> RSPWEENFSRSYPCDEKKQNDSVIAECSNRRLQEVPQTVGKYVTELDLSDNFITHITNESFQGLQNLTKINLNHNPNVQHQNGNPGIQSNGLNITDGAFLNLKNLRELLLEDNQLPQIPSGLPESLTELSLIQNNIYNITKEGISRLINLKNLYLAWNCYFNKVCEKTNIEDGVFETLTNLELLSLSFNSLSHVPPKLPSSLRKLFLSNTQIKYISEEDFKGLINLTLLDLSGNCPRCFNAPFPCVPCDGGASINIDRFAFQNLTQLRYLNLSSTSLRKINAAWFKNMPHLKVLDLEFNYLVGEIASGAFLTMLPRLEILDLSFNYIKGSYPQHINISRNFSKLLSLRALHLRGYVFQELREDDFQPLMQLPNLSTINLGINFIKQIDFKLFQNFSNLEIIYLSENRISPLVKDTRQSYANSSSFQRHIRKRRSTDFEFDPHSNFYHFTRPLIKPQCAAYGKALDLSLNSIFFIGPNQFENLPDIACLNLSANSNAQVLSGTEFSAIPH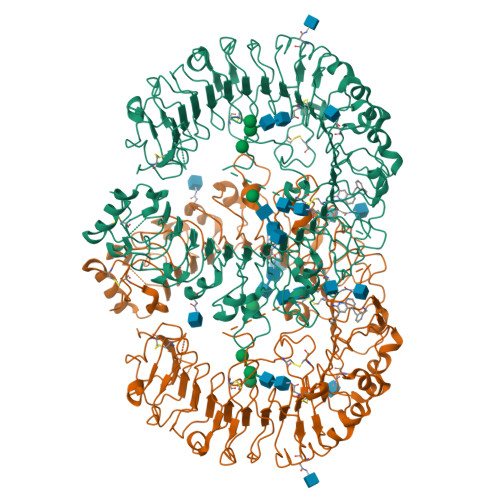VKYLDLTNNRLDFDNASALTELSDLEVLDLSYNSHYFRIAGVTHHLEFIQNFTNLKVLNLSHNNIYTLTDKYNLESKSLVELVFSGNRLDILWNDDDNRYISIFKGLKNLTRLDLSLNRLKHIPNEAFLNLPASLTELHINDNMLKFFNWTLLQQFPRLELLDLRGNKLLFLTDSLSDFTSSLRTLLLSHNRISHLPSGFLSEVSSLKHLDLSSNLLKTINKSALETKTTTKLSMLELHGNPFECTCDIGDFRRWMDEHLNVKIPRLVDVICASPGDQRGKSIVSLELTTCVSDVTEFLVPR> GAMAPATCEKPKFLEYKTCVGDLTVVIAKALDEFKEFCIVNAANEHMTHGSGVAKAIADFCGLDFVEYCEDYVKKHGPQQRLVTPSFVKGIQCVN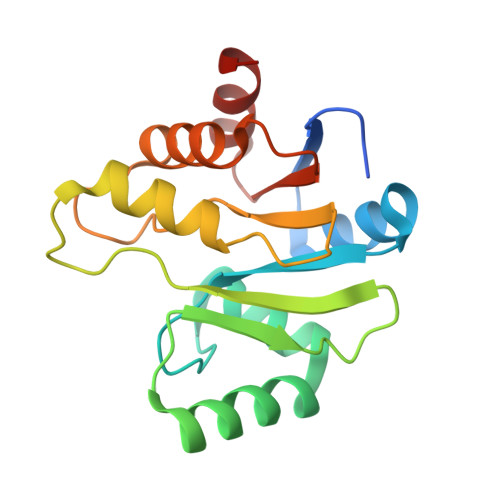NVVGPRHGDNNLHEKLVAAYKNVLVDGVVNYVVPVLSLGIFGVDFKMSIDAMREAFEGCTIRVLLFSLSQEHIDYFDVTCK> GPVDVKLEFVLYRKNVTLAELEAMGQQQLLSLPTNAELNVEIMANGVLLGNGELVQM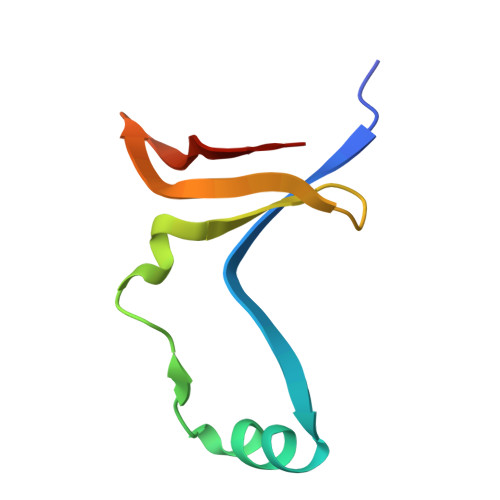NDTLGVEIHEWLS> ETVNVTVGQV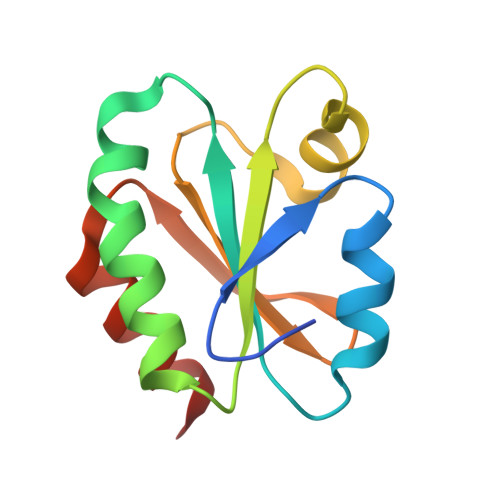TEVDKDTFWPIVKAAGDKIVVLDMYTQWCGPSKVIAPKYKELSEKYQDMVFLKLDCNQDNKPLAKELGIRVVPTFKILKDNKVVKEVTGAKYEDLLAAIEAARSG>[4x]MRIPLVGKDSIESKDIGFTLIHEHLRVFSEAVRQQWPHLYNEDEELRNAVNEVKRAMQFGVKTIVDPTVMGLGRDIRFMEKVVKATGINLVAGTGIYIYIDLPFYFLNRSIDEIADLFIHDIKEGIQGTLNKAGFVKIAADEPGITKDVEKVIRAAAIANKETKVPIITHSNAHNNTGLEQQRILTEEGVDPGKILIGHLGDTDNIDYIKKIADKGSFIGLDRYGLDLFLPVDKRNETTLRLIKDGYSDKIMISHDYACTIDMGTAKPEYKPKLAPRWSTTLIFEDTIPFLKRNGVNEEVIATIFKENPKKFFS

Phosphotriesterase-like Lactonases (PLLs) are appealing candidates, being natural lactonases endowed with promiscuous phosphotriesterase activity. PTEs and PLLs belong to the amidohydrolase superfamily, and share the same (β/α)8 barrel topology. SsoPox exhibits high acyl-homoserine lactones and oxo-lactones hydrolysis abilities, and promiscuous, low phosphotriesterase activity. SsoPox is a very appealing candidate for the bioremediation of phosphotriesters because of its unique thermal stability, and its ability to resist aging, solvent and protease treatments.

Of them, the most active variants, αsA1 (C258L-I261F-W263A), αsA6 (F46L-C258A-W263M-I280T), αsB5 (V27A-I76T-Y97W-Y99F-L130P-L226V), αsC6 (L72I-Y99F-I122L-L228M-F229S-W263L), and αsD6 (V27A-Y97W-L228M-W263M) were subject to kinetic and structural characterization. Although the active sites of the improved variant structures superpose well onto the wt-structure, all selected mutants display altered loop 8 conformations. Notably, mutant αsA6 was crystallized in two different conformations: one in which loop 8 adopts a wt-like conformation, referred to as closed conformation (CC), and another one where loop 8 is unfolded, referred to as open conformation (OC). Interestingly, variants αsA6 and αsC6 exhibit enhanced lactonase activity against γ- and δ-lactones, while αsA1, αsB5 and αsD6 show reduced lactonase catalytic efficiencies. This emphasizes the fact that the improvement of the phosphotriesterase activity does not necessarily compromise the cognate, lactonase activity of the enzyme.> MGSSHHHHHHSSGLVPRGSHMASISKDFTNLLNTLIDGQIGAASRQTEWFNMSPDERTDYIKQVDERLQEMQQSTLSVLAAQHFQMQDNPVSVGDQLQTLQKRRQQMTDVPGTPAINAYKQQLDRDILLYRRQQTAMTHFDSTWRKVLVMLGPDDSKPLNATTLRENAVDKQAKLDTEIKRLEQQLTIQVADSTFSQKYVTLFSELQAYKDVNARYNALLKASATEEAAALGALTKVPQASDDLPVNISLLMMEERPGYIRMNVALVNASTDGRFKDFFLENGRLVVLTDGVLNFSFGTAARSLAWQQQYRLKSEPPSFRSPTYTPIRSVLVKTEFVEKYFANYLVSESTLRGGFKAQLLGNGRKMLLTSVDRKVPNQIGIQVSGQAPNTTITREVPLASALSDLINQNADIASFRTIGLEGFRQSSYHPDRDGLFVNIHELERSVGFAGRQYLLEMPQDNDYLSATPFGVMSVDGDKVSSSHLSKAQTDTLYQYNAAFFEKLEQLRSGGMKASRLFEGSIERTAFVQQLVRLLERNHITPAGVLAPEYPRDNMRDIKGNNLNKVLWEQAFAASVWRSRDNDPLLFRLATRLVKNPAVVKVLQNGYVQSDIAQARELLAPLYEQWRTRAVEAETQRVASANAAQHPSNPKVHVFDQAEVERSLDDKLLILLLTGPQSLEGTDVQLRPMVEAALLSNEGRSLRKQILFHALRPVADSFSKAAAPVNPHAELGVGKIMINNRLNQPDPYLILNTSSEEQAYRDGSYLIKDDKYRSYNQFRPDFKNDATRYMNDLDTPFVGGISGTTQTVSNVLTELFGGALSVKQYWQFQMANAAFMIRNGYHSFFETFYVAARYEPEGADSIGKEMLQMFDKYRVEGSKKALQGKLYDGVMARVLPIINQGLSAADEFHPPRFTRIGPRPALLGQAVKDLELKAGLTSVGDGFEPRQGSADIHQFVTDPVLFAKTHTVSAEALVRSGRLPAEGSAQLVKVGSGLYELEYTEQSANDISSSSIPAYFLGYNGPNQANAVPAYVDIPKRTIAGNFLFTGTLSGGSLVVTSLDANTFRVYHDGRVNSSLLYDNVVMAVDYKDYQIAGTAEGLAAAYMQYVNHEWQLVLQRQEYQRDGQMLRLRLRDDEEPLSIQVADSQVVERNQAQFVAYREQIHQQLKKVATQFEVSISGVSDGVYTEGEFSPDHPAIAAWAKLCAEVYDRINADTKQLVDKRNKLYENRRNTIRRDLINQQIKQLNITLEYYKAQYDTVLREAGFVEQSWLWQQIKAKNGSAAVVRIDDTAIQGGGKQRTDSVGERYAISEAYQRGARGTGFSDGLRNFREIEIPGVDDKMSALEMKRLFLEGKLTSEQQGALSGRITETSRAEYIDKVLRQTAVFSEDFHDAGSVFDRLVPQDFYLSLVGDRSGGRAYPLVRAMTVALASGGEAGINSLVQKLFFASADPQAGSSTLLRNSLIKLHSNVEAVQASTELGQFGLSEVVSRLAATTGTSMFALNTQNHSMMVGSTVTTEGRRYYFYDPNVGIFAFDNTKSLSRAMEQHLVGRRLAVHYGSFGSKSAPAFNLIEIDTGKMAEVPVGNGLNVADLTRFEELSSVIGQRRQVEQVMSAQERITEDLQLSTALQAFDAEQWGARFEAASTRLAQEHQLDSRWLPIIATTEEQGEGRYRVQFINRDQPEQTRWLDTDDSTFVEFRRFVDEHMSVLNEHFTLESGRMRPRGGVGEAAPVDGLNAGFAVQALIQWFSDKNRHDAANGMASPDLATALKVHSYLNFVQMVHGGVQDVIKVTALVRTALRGEVVAAQTSFKEFALSLGHTVNEGVGVLFGGAMIGLDAYELAHAENDVQKAVFGTQLAFDSASFVTGAAGIGAGLVGASTAGAVLGGAGVILGGLAVGFTALAQAFGAVAEDAKAVGRYFDTVDKAYKGNGYRYDNEKQVLVPLAGAVIKTLDLSKNQIDFDSQYIYRTHSGSTGSGKINYFFWVGDFPRMVHDRGQAIEVRSGIGYKDVSRPLEHGDSNVVILPGTPKSYISYEYMLLPGATTRHDAGFDVIRRLEEDKRFDYDFYIFPGEETIRRIHHEYVDTPIEVVLDQRNRQLVAPELPKELHGFLCYEIKGAGGEYLIGLNEGAKVNLTSDVASTWIIDSSQLASDSISVSKDQLLVGEKGKEVVVKLYLAQNSQVLVVNGKGEVRKVDFTSLTAQVISEDASKWQVPGQQIEQHLSDLAKAHQLHGQYVVVENYRHQGRDVGRAFYDVTKDRMLFTDTTNEQAKRAQLGAVMGDYAYFYDADNAVAWRVDIATGQVDAQFEPWFNQNAGHISRFWQEGDVVYLARRYRLKEREAELGYRIIGDRMELVSAVGDDALLQLSARIGRHGDELEAILQGYRSNSTQRGTLMYTLGARLIQPTSAALVTVFGVDAAGVPHRYWIRTSDGTLIKPNLAPPADQTLHFEAHEQTRSAWQIPADLVLAGSMPLLGGKEVFFFYSKEQKTLFRQEGPGQEVLDANQPSALRVTTPALTNVINLNGHLVVVTEDGRVARLDALGQLSYAAVNEHWLKGRIHWWQDLTSVTDGRATLAVFGVKDTDGKSLLPVWYHNGQVVVASAALQDKHPQFLGFEVDGSSARLFEPASGKLYRQPAMTADALAAAFGTDEVLEASAQLPAANELEPELHLKAAEQVDAGLRLTTVKGEILLRTHDGKLQLVAVDKDWQQDNLVRLSQALAEVAGQWRVKGVLTLQGDDTQGWFDVGSGQVFSIGGIPATDNLRFIGIAVGKKGAYVYNPTDQMLYQVKESGAQKLNHYADVERIGSSLLLQDGGKGDLSPMLIAGVDSVVLHGGAGSDTYRLSQTMWSYYRTVVIDNDDPNQVLDRLIILAVDAEKIFVSRHEDDLMLTDSVNGTVLVIRKVFGSQAVTHRHLQIDLEGSSSVISVDHLVKGFTR

The bacterial Makes caterpillars floppy 1 (Mcf1) toxin promotes apoptosis in insects, leading to loss of body turgor and death. The structure reveals that Mcf1 is divided into an N-terminal head region and a C-terminal tail region. The head contains an N-terminal effector domain (NED), an activator-binding domain (ABD), and a protease effector domain (PED). The tail consists of two putative translocation and three putative receptor-binding domains.

To test the role of the C-terminal region of Mcf1 in the autoprocessing reaction, we purified a Mcf1 mutant devoid of 15 C-terminal amino acids (Δ15C) and incubated it with Arf3 in vitro. Strikingly, the autocleavage reaction proceeded several times faster than with the wild-type toxin and yielded the same fragments. This result demonstrates that the C-terminus of Mcf1 is a potential regulatory element that prevents autoprocessing of Mcf1 prior to its translocation into the target cell. To decipher the molecular mechanism of the activation process, we analyzed the Mcf1-Arf3 interaction by cryo-EM and single particle analysis. To obtain a stable complex, we used the C1397A Δ15C variant of Mcf1 to make sure that the protease is inactive and the C-terminus does not interfere with the interaction (see above) and determined structures of the Mcf1 variant in the absence and presence of Arf3. During particle selection and 2D classification, we noticed in both datasets that the Mcf1 head domain was clearly visible, while the tail domain was absent in most 2D classes or blurry in others. This is in contrast to the single particle analysis of the wild type and suggests, that the removal of the last 15 amino acids destabilizes the neck regions leading to a high flexibility between the head and tail. Therefore, we only concentrated on the heads for the following analysis. During 3D refinement and classification, we noticed that the heads were also very heterogenous and the ABD was missing in most classes of Mcf1C1397A Δ15C. Nevertheless, we managed to determine a cryo-EM structure of the complete head of Mcf1C1397A Δ15C in absence of Arf3 at 3.5 Å resolution. The comparison of the Mcf1C1397A Δ15C-Arf3 structure with Mcf1C1397A Δ15C, however, showed that the position of the protease domain is not altered and the cleavable linker is more or less in the same position, indicating that Arf3 binding does not induce direct conformational changes.> DTPEPPLHNFYCSKLLDLVFLLDGSSMLSEAEFEVLKAFVVGMMERLHISQKRIRVAVVEYHDGSRAYLELKARKRPSELRRITSQIKYTGSQVASTSEVLKYTLFQIFGKIDRPEASHITLLLTASQEPPRMARNLVRYVQGLKKKKVIVIPVGIGPHASLKQIRLIEKQAPENKAFLLSGVDELEQRRDEIVSYLC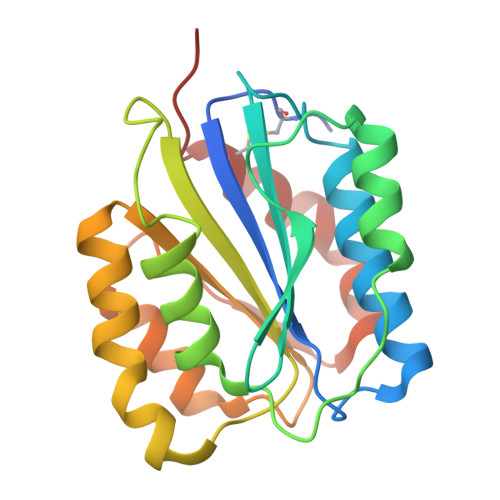DLAPEAPAPT> ETGICKGCLSCSKDNGCSRCQQKLFFFLRREGMRQYGECLHSCPSGYYGHRAPDMNRCARCRIENCDSCFSKDFCTKCKVGFYLHRGRCFDECPDGFAPLDE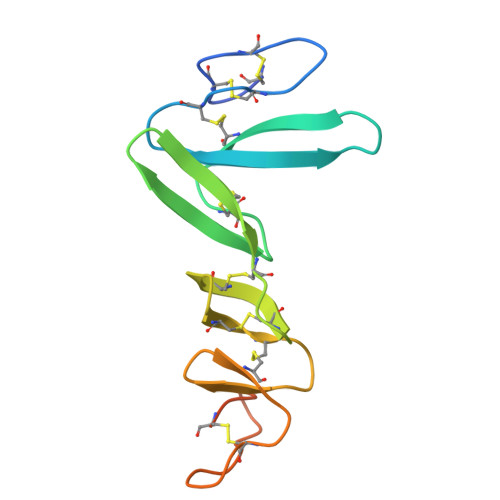TMECVEGTHHHHHHHHHH>VTKTITEQRAEVRIFAGNDPAHTATGSSGISSPTPALTPLMLDEATGKLVVWDGQKAGSAVGILVLPLEGTETALTYYKSGTFATEAIHWPESVDEHKKAN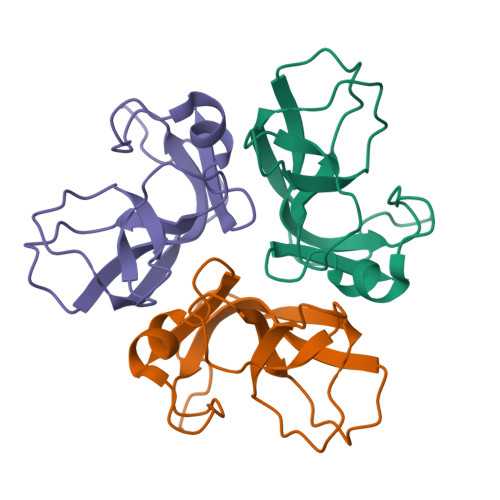AFAGSALSHAALP[4x]>[4x]MGSVRTNRYSIVSSEEDGMKLATMAVANGFGNGKSKVHTRQQCRSRFVKKDGHCNVQFINVGEKGQRGGRNETLVFSHNAVIAMRDGKLCLMWRVGNLRKSHLVEAHVRAQLLKSRITSEGEYIPLDQIDINVGFDSGIDRIFLVSPITIVHEIDEDSPLYDLSKQDIDNADFEIVVILEG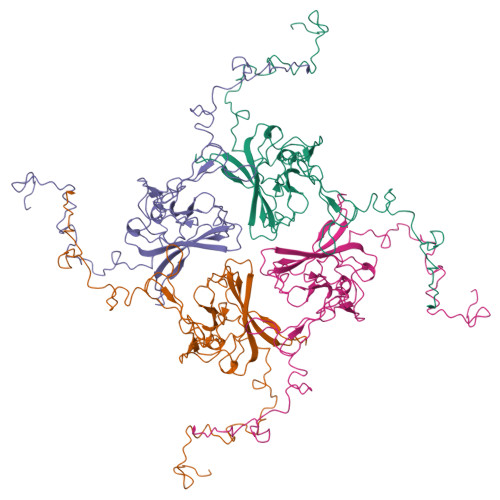MVEATAMTTQCRSSYLANEILWGHRYEPVLFEEKHYYKVDYSRFHKTYEVPNTPLCSARDLAEKKYILSNANSFCYENEVALTSKEEEEDSENGVPESTSTDSPPGIDLHNQASVPLEPRPLRRESEI> MEGLAGYVYKAASEGKVLTLAALLLNRSESDIRYLLGYVSQQGGQRSTPLIIAARNGHAKVVRLLLEHYRVQTQQTGTVRFDGYVIDGATALWCAAGAGHFEVVKLLVSHGANVNHTTVTNSTPLRAACFDGRLDIVKYLVENNANISIANKYDNTCLMIAAYKGHTDVVRYLLEQRADPNAKAHCGATALHFAAEAGHIDIVKELIKWRAAIVVNGHGMTPLKVAAESCKADVVELLLSHADCDRRSRIEALELLGASFANDRENYDIIKTYHYLYLAMLERFQDGDNILEKEVLPPIHAYGNRTECRNPQELESIRQDRDALHMEGLIVRERILGADNIDVSHPIIYRGAVYADNMEFEQCIKLWLHALHLRQKGNRNTHKDLLRFAQVFSQMIHLNETVKAPDIECVLRCSVLEIEQSMNRVKNISDADVHNAMDNYECNLYTFLYLVCISTKTQCSEEDQCKINKQIYNLIHLDPRTREGFTLLHLAVNSNTPVDDFHTNDVCSFPNALVTKLLLDCGAEVNAVDNEGNSALHIIVQYNRPISDFLTLHSIIISLVEAGAHTDMTNKQNKTPLDKSTTGVSEILLKTQMKMSLKCLAARAVRANDINYQDQIPRTLEEFVGFH;> GGGSGGGSKKHSLDLLSKERELNGKLRHLSP

We recently discovered that FEM1B, a substrate receptor of Cullin 2-RING ligase (CRL2), recognizes C-degrons containing a C-terminal proline. By solving several cryo-EM structures of CRL2FEM1B bound to different C-degrons, we elucidate the dimeric assembly of the complex. Furthermore, we reveal distinct dimerization states of unmodified and neddylated CRL2FEM1B to uncover the NEDD8-mediated activation mechanism of CRL2FEM1B. Our research also indicates that, FEM1B utilizes a bipartite mechanism to recognize both the C-terminal proline and an upstream aromatic residue within the substrate.

Due to the limited resolution of C-degron peptides observed in all solved cryo-EM structures, we performed local refinement for the N8CRL2FEM1B dimerS1 to obtain a 3.55 Å resolution structure of the FEM1B-CCDC89 subcomplex. For convenience, the peptide is numbered from the C-terminus, with the last Pro being Pro-1, the penultimate Ser being Ser-2, etc. Most residues of CCDC89 are visible in the structure except for the five central residues (−12RELNG−8), probably due to their intrinsic flexibility. The C-terminal  region of the peptide adopts a 310 helix structure and occupies the CDK5R1 Arg/C-degron binding site of FEM1B, which is formed by ANK3-4. Pro-1 is accommodated by the same FEM1B pocket that has been reported to recognize the arginine at C-end. The main chain carbonyl group of Pro-1 is hydrogen bonded to the side chains of Ser122 and Arg126 of FEM1B, and its side chain forms hydrophobic interactions with Tyr84, Trp93, and Phe130. The main chain carbonyl groups of Ser-2 and Leu-3 are hydrogen bonded to the side chains of Arg126 and Tyr84, respectively, with Leu-3 forming hydrophobic interactions with Ile160, Tyr163, and Phe193. The N-terminal portion of the CCDC89 peptide, −22KHSLDLLSKE−13, adopts an α-helical conformation and interacts with TPR3, TPR4, and a 310 helix insertion in ANK8. Specifically, His-21 is positioned in a hydrophobic pocket composed of Val391, Phe501, and His502. Additionally, the imidazole ring and main chain nitrogen group of His-21 form hydrogen bonds with the side chains of Gln394 and Asp356, respectively.> MSYAVAGALQAAVYQQLRADAVLAALVGTAVYDAVPPGPLAGTYVSLGPEDVADASDKTGAGAVHDFVISVITDAAGFATAKAAAAAVSDALVGADLVLSRGRLVGLWFLRAKARRVEKADMRR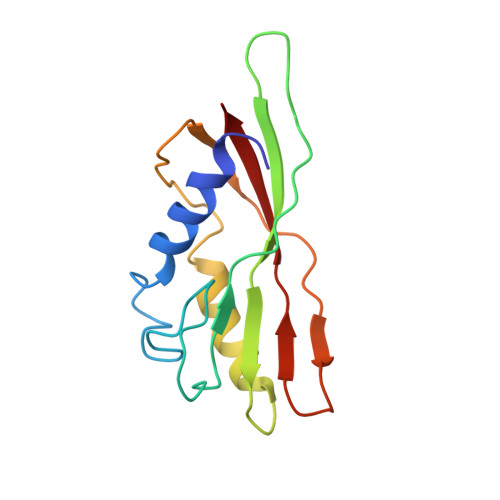IDLVFRARVEG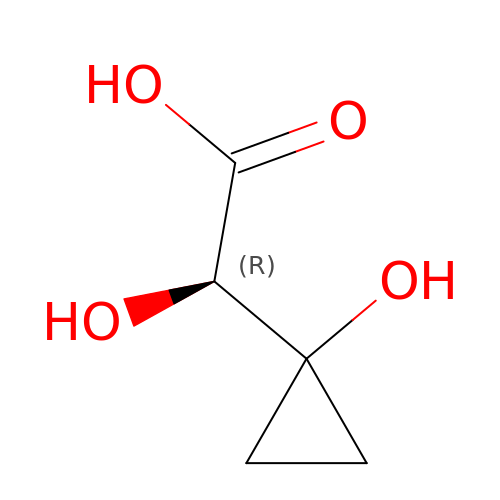(2R)-2-oxidanyl-2-(1-oxidanylcyclopropyl)ethanoic acid | C5 H8 O4 | XIFMBZFYSIRQIK-VKHMYHEASA-N> PKPAPRYNIGLRPAPKRQNVGGQFLATQKHYARELWYKRQYYSTRPFAIQKHMGSTPRILLDRTLWRS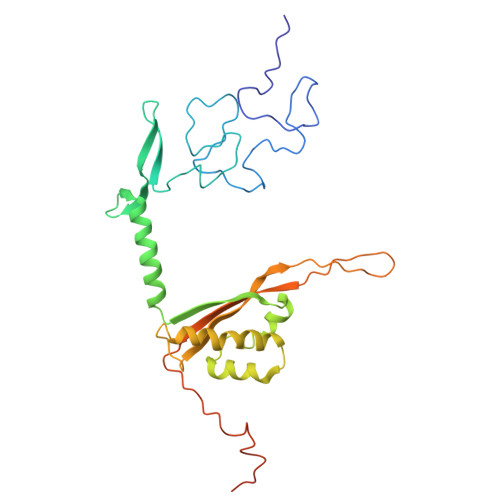CWLTKSNLPDVNRWEKVVNSQRVTEDRWALVEEDGVMYQVNWKMYCERLETELQKAQDQLPQYSFMMKAVPSAWKKLDIELSVLRGLSVREAMAQCKLSPRKGHMAVFRALEVAQQGAEGKGLDKEHLRIAYITCMPGPTDKQVDIRSRGYYAWKTKKSSHLLLTLAEDPEMVLPDRTAIPYASLMTMKRAGLRTEPTMLDVPAITAEGI>[2x]SIDKNFWQGKRVFVTGHTGFKGSWLSLWLTEMGAIVKGYALDAPTVPSLFEIVRLNDLMESHIGDIRDFEKLRSSIAEFKPEIVFHMAAQPLVRLSYEQPIKTYSTNVMGTVHLLETVKQVGNIKAVVNITSDKCYDNREWVWGYRENEPMGGYDPYSNSKGC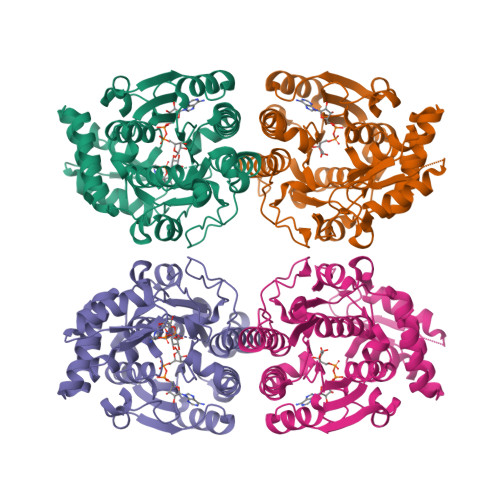AELVASAFRNSFFNPANYEQHGVGLASVRAGNVIGGGDWAKDRLIPDILRSFENNQQVIIRNPYSIRPWQHVLEPLSGYIVVAQRLYTEGAKFSEGWNFGPRDEDAKTVEFIVDKMVTLWGDDASWLLDGENHPHEAHYLKLDCSKANMQLGWHPRWGLTETLSRIVKWHKAWIRGEDMLICSKREISDYMSATTR> MWGLQPPTSIPPPPPPTELTPSTYPAMVNGYPPPAASAQSCSSSGGQSELYMPLQRVMAPTGGRNSIKYRDYTPCRNTTKLFYVDNKASDIDTYNK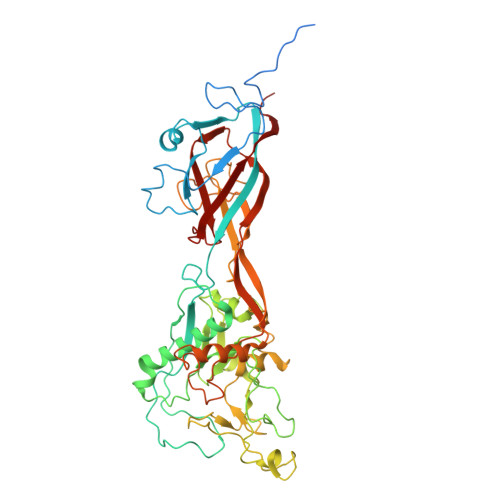DANHSNFRTTVIHNQDLDADTAATESIQLDNRSCWGGDLKTAVRTNCPNVSSFFQSNSVRVRMMWKRDPPTSTAPPSAVGSGYSVPGAQYKWYDLTVPEGNYALCELIDLLNEGIVQLYLSEGRQNNVQKSDIGVKFDTRNFGLLRDPVTGLVTPGTYVYKGYHPDIVLLPGCAIDFTYSRLSLLLGIGKREPYSKGFVITYEDLQGGDIPALLDLDSVDVNDADGEVIELDNAAPLLHDSAGVSYNVIYDQVTGKPVTAYRSWMLAYNVPNSQANQTTLLTVPDMAGGIGAMYTSLPDTFIAPTGFKEDNTTNLCPVVGMNLFPTYNKIYYQAASTYVQRLENSCQSATAAFNRFPENEILKQAPPMNVSSVCDNQPAVVQQGVLPVKSSLPGLQRVLITDDQRRPIPYVYKSIATVQPTVLSSATLQ> MGSDKIHHHHHHTHSVETPYGSVTFTVYGTPKPKRPAIFTYHDVGLNYKSCFQPLFRFGDMQEIIQNFVRVHVDAPGMEEGAPVFPLGYQYPSLDQ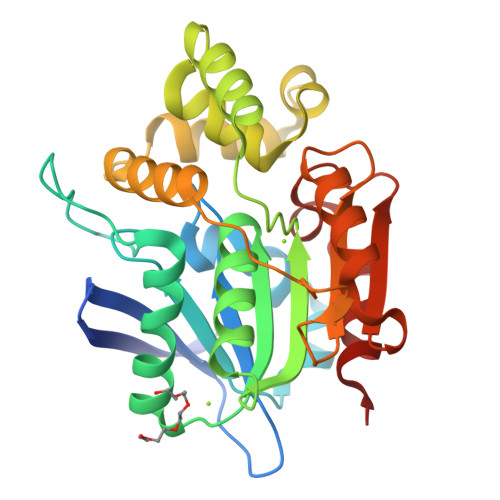LADMIPCILQYLNFSTIIGVGVGAGAYILSRYALNHPDTVEGLVLINIDPNAKGWMDWAAHKLTGLTSSIPDMILGHLFSQEELSGNSELIQKYRGIIQHAPNLENIELYWNSYNNRRDLNFERGGETTLKCPVMLVVGDQAPHEDAVVECNSKLDPTQTSFLKMADSGGQPQLTQPGKLTEAFKYFLQG> MSNLSGTDKSVILLMTIGEDRAAEVFKHLSTREVQALSTAMANVRQISNKQLTDVLSEFEQEAEQFAALNINANEYLRSVLVKALGEERASSLLEDILETRDTTSGIETLNFMEPQSAADLIRDEHPQIIATILVHLKRSQAADILALFDERLRHDVMLRIATFGGVQLAELTEVLNGLLDGQNLKRSKMGGVRTAAEIINLMKTQQEEAVITAVREFDGELAQKIIDEMFLFENL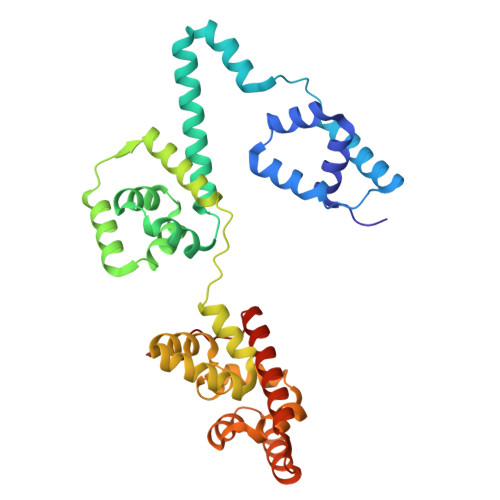VDVDDRSIQRLLQEVDSESLLIALKGAEPPLREKFLRNMSQRAADILRDDLANRGPVRLSQVENEQKAILLIVRRLAETGEMVIGSGEDTYV> GLSIGIVGATGQVGQVMRTLLDERDFPASAVRFFASARSQGRKLAFRGQEIEVEDAETADPSGLDIALFSAGSAMSKVQAPRFAAAGVTVIDNSSAWRKDPDVPLVVSEVNFERDAHRRPKGIIANPNCTTMAAMPVLK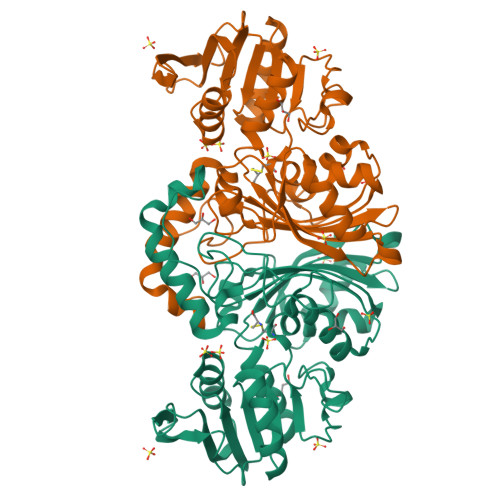VLHDEARLVRLVVSSYQAVSGSGLAGVAELAEQARAVIGGAEQLVYDGGALEFPPPNTYVAPIAFNVVPLAGSLVDDGSGETDEDQKLRFESRKILGIPDLLVSGTCVRVPVFTGHSLSINAEFAQPLSPERARELLDGATGVQLVDVPTPLAAAGVDESLVGRIRRDPGVPDGRGLALFVSGDNLRKGAALNTIQIAELLTADL> GSDEKRLHFGNGHLKLPGLRTFVDPHTFEDPTQTVHEFAKELDATNISIDKVVGAGEFGEVCSGRLKLPSKKEISVAIKTLKVGYTEKQRRDFLGEASIMGQFDHPNIIRLEGVVTKSKPVMIVTEYMENGSLDSFLRKHDAQFTVIQLVGMLRGIASGMKYLSDMGFVHRDLAARNILINSNLVCKV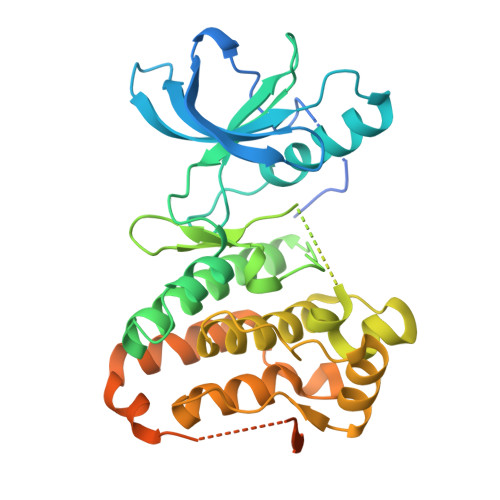SDFGLSRVLEDDPEAAYTTRGGKIPIRWTSPEAIAYRKFTSASDVWSYGIVLWEVMSYGERPYWEMSNQDVIKAVDEGYRLPPPMDCPAALYQLMLDCWQKDRNNRPKFEQIVSILDKLIRNPGSLKIITSAAARPSNLLLDQSNVDITTFRTTGDWLNGVWTAHCKEIFTGVEYSSCDTIAKIS> GAQNRNTSICRLGFTYDISQSKNWGNNKPVIKSIIPYSSAEQAGIKKYDVIEEINGVPVTEVSVDEIPQLLNPAGRNDVLLTISNLSSPSKQVLVKKDCKKSNAITEDQLASAYAMYSLETTNEQEFVCPFKTTVTSDGVDFGNFKTFAFSTIDENNRKLETVINECIENELTKKGLTVDIAKPDLLIQTFYFFDKNPNYLGANKVLVEKEPTYRYNFSHSKMEKFPFLNYAAAEAEAEYLLQFGIRIIDQKDIPGRVLWECEANELLEDSYRLDEYARVHVPLMCMQYPYTKYGRNVPFKVSKKTYNYTGISYDIDKLDQVVDVDRNSPAYAAGIRPRDIIEKIGRHKMDHSAEEFSSAYKRFITNTMQYRDPKTMFTDANGFKYCMFWDVFKYPQ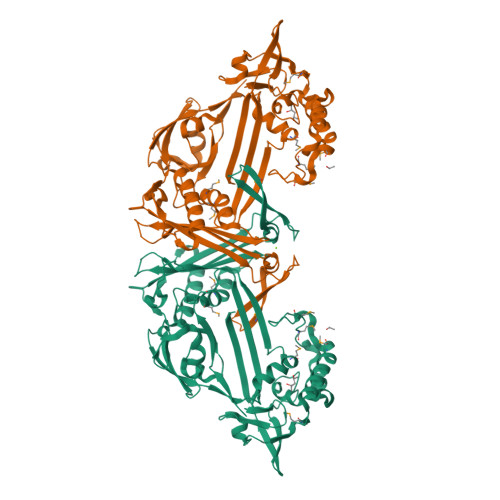IADASQSSDYLPAFSYLYYFAPYINPSGNNACTFNIKRGKTKLEVIIRPTIRSEVTVEIK>[2x]SMKIDVVTIFPEYLQPVRQSLPGKAIDAGLVDVAVHDLRRWTHDVHKSVDDSPYGGGPGMVMKPTVWGDALDEICTSETLLVVPTPAGYPFTQETAWQWSTEDHLVIACGRYEGIDQRV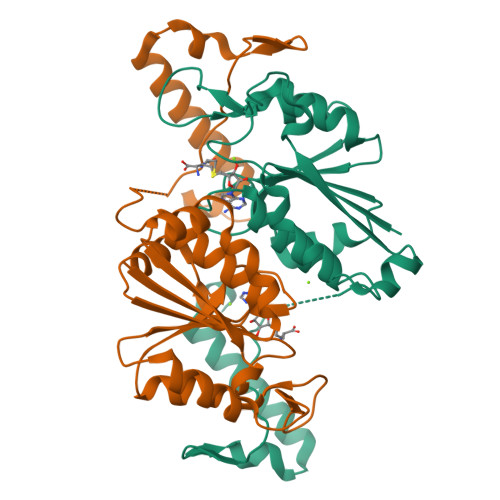ADDAATRMRVREVSIGDYVLNGGEAAALVIIEAVLRLVPGVLGNALSAQEDSHSEGMASLLEGPSYTRPPSWRGMDVPPVLLSGDHAKIAAWRAEQSRQRTIERRPDLLGFDSP2-sulfanylbenzoic acid | C7 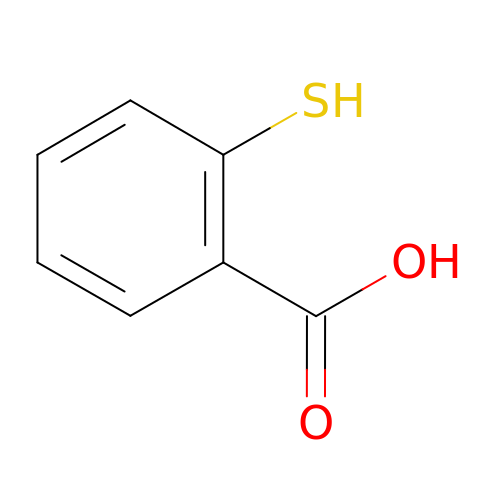H6 O2 S | NBOMNTLFRHMDEZ-UHFFFAOYSA-N> GPKITLLTLIKTAEHWARQDIRTIEDSKLRALLTLCAVMTRKFSKSQLSLLCETHLRREGLGQDQAEPVLEVYQRLHSDKGGSFEAAL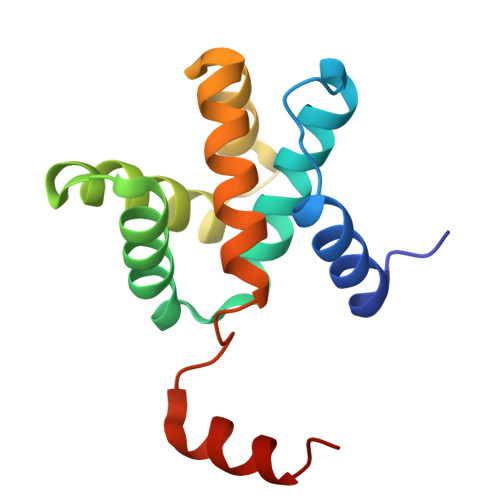WQQWDRQSLIMFITAFLNIALQLPCESSAVVVSGLRTLVPQ> GPVWRKHYITYRINNYTPDMNREDVDYAIRKAFQVWSNVTPLKFSKINTGMADILVVFARGAHGDFHAFDGKG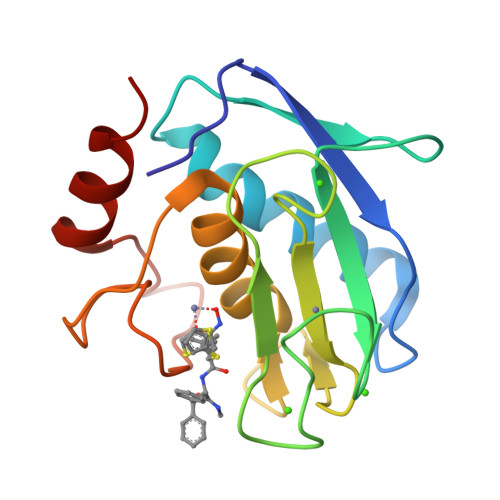GILAHAFGPGSGIGGDAHFDEDEFWTTHSGGTNLFLTAVHAIGHSLGLGHSSDPKAVMFPTYKYVDINTFRLSADDIRGIQSLYG>MSKVAMVTGGAQ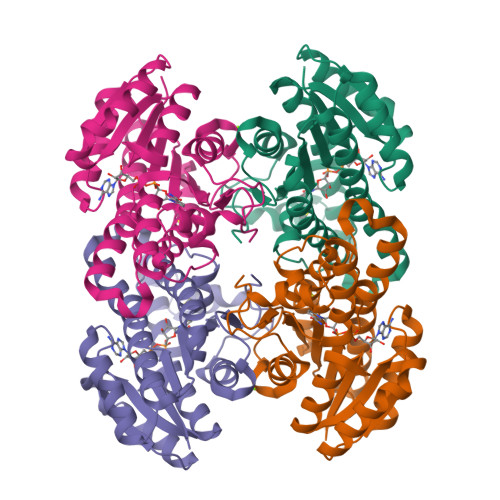GIGRGISEKLAADGFDIAVADLPQQEEQAAETIKLIEAADQKAVFVGLDVTDKANFDSAIDEAAEKLGGFDVLVNNAGIAQIKPLLEVTEEDLKQIYSVNVFSVFFGIQAASRKFDELGVKGKIINAASIAAIQGFPILSAYSTTKFAVRGLTQAAAQELAPKGHTVNAYAPGIVGTGMWEQIDAELSKINGKPIGENFKEYSSSIALGRPSVPEDVAGLVSFLASENSNYVTGQVMLVDGGMLYN[8x]> SKKRQWALEDFEIGRPLGKGKFGNVYLAREKQSKFILALKVLFKAQLEKAGVEHQLRREVEIQSHLRHPNILRLYGYFHDATRVYLILEYAPLGTVYRELQKLSKFDEQRTATYITELANALS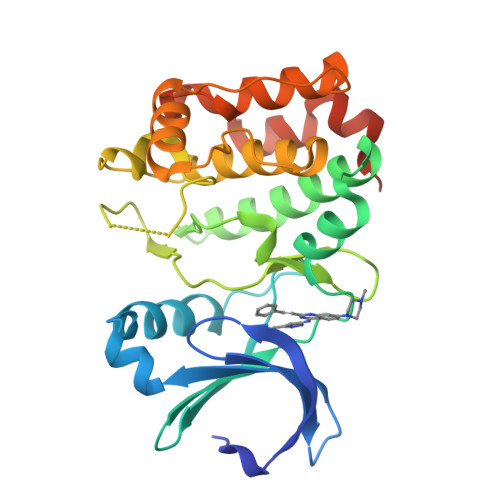YCHSKRVIHRDIKPENLLLGSAGELKIADFGWSVHAPSSRRTTLCGTLDYLPPEMIEGRMHDEKVDLWSLGVLCYEFLVGKPPFEANTYQETYKRISRVEFTFPDFVTEGARDLISRLLKHNPSQRPMLREVLEHPWITANSSKPSNCQNKESASKQS>MNLLRRSGKRRRSESGSDSFSGSGGDSSASPQFLSGSVLSPPPGLGRCLKAAAAGECKPTVPDYERDKLLLANWGLPKAVLEKYHSFGVKK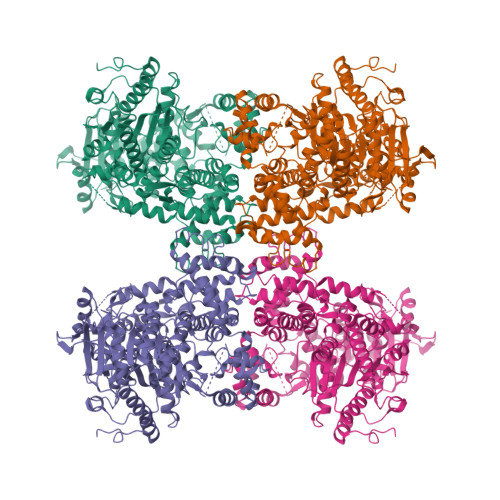MFEWQAECLLLGQVLEGKNLVYSAPTSAGKTLVAELLILKRVLEMRKKALFILPFVSVAKEKKYYLQSLFQEVGIKVDGYMGSTSPSRHFSSLDIAVCTIERANGLINRLIEENKMDLLGMVVVDELHMLGDSHRGYLLELLLTKICYITRKSASCQADLASSLSNAVQIVGMSATLPNLELVASWLNAELYHTDFRPVPLLESVKVGNSIYDSSMKLVREFEPMLQVKGDEDHVVSLCYETICDNHSVLLFCPSKKWCEKLADIIAREFYNLHHQAEGLVKPSECPPVILEQKELLEVMDQLRRLPSGLDSVLQKTVPWGVAFHHAGLTFEERDIIEGAFRQGLIRVLAATSTLSSGVNLPARRVIIRTPIFGGRPLDILTYKQMVGRAGRKGVDTVGESILICKNSEKSKGIALLQGSLKPVRSCLQRREGEEVTGSMIRAILEIIVGGVASTSQDMHTYAACTFLAASMKEGKQGIQRNQESVQLGAIEACVMWLLENEFIQSTEASDGTEGKVYHPTHLGSATLSSSLSPADTLDIFADLQRAMKGFVLENDLHILYLVTPMFEDWTTIDWYRFFCLWEKLPTSMKRVAELVGVEEGFLARCVKGKVVARTERQHRQMAIHKRFFTSLVLLDLISEVPLREINQKYGCNRGQIQSLQQSAAVYAGMITVFSNRLGWHNMELLLSQFQKRLTFGIQRELCDLVRVSLLNAQRARVLYASGFHTVADLARANIVEVEVILKNAVPFKSARKAVDEEEEAVEERRNMRTIWVTGRKGLTEREAAALIVEEARMILQQDLVEM[4x]> MDKYDKNVPSDYDGLFQKAADANGVSYDLLRKVAWTESRFVPTAKSKTGPLGMMQFTKATAKALGLRVTDGPDDDRLNPELAINAAAKQLAGLVGKFDGDELKAALAYNQGEGRLGNPQLEAYSKGDFASISEEGRNYMRNLLDVAKSPMAGQLETFGGITPKGKGIPAEVGLAGIGHKQKVTQELPESTSFDVKGIEQEATAKPFAKDFWETHGETLDEYNSRSTFFGFKNAAEAELSNSVAGMAFRAGRLDNGFDVFKDTITPTRWNSHIWTPEELEKIRTEVKNPAYINVVTGGSPENLDDLIKLANENFENDSRAAEAGLGAKLSAGIIGAGVDPLSYVPMVGVTGKGFKLINKALVVGAESAALNVASEGLRTSVAGGDADYAGAALGGFVFGAGMSAISDAVAAGLKRSKPEAEFDNEFIGPMMRLEARETARNANSADLSRMNTENMKFEGEHNGVPYEDLPTERGAVVLHDGSVLSASNPINPKTLKEFSEVDPEKAARGIKLAGFTEIGLKTLGSDDADIRRVAIDLVRSPTGMQSGASGKFGATASDIHERLHGTDQRTYNDLYKAMSDAMKDPEFSTGGAKMSREETRYTIYRRAALAIERPELQKALTPSERIVMDIIKRHFDTKRELMENPAIFGNTKAVSIFPESRHKGTYVPHVYDRHAKALMIQRYGAEGLQEGIARSWMNSYVSRPEVKARVDEMLKELHGVKEVTPEMVEKYAMDKAYGISHSDQFTNSSIIEENIEGLVGIENNSFLEARNLFDSDLSITMPDGQQFSVNDLRDFDMFRIMPAYDRRVNGDIAIMGSTGKTTKELKDEILALKAKAEGDGKKTGEVHALMDTVKILTGRARRNQDTVWETSLRAINDLGFFAKNAYMGAQNITEIAGMIVTGNVRALGHGIPILRDTLYKSKPVSAKELKELHASLFGKEVDQLIRPKRADIVQRLREATDTGPAVANIVGTLKYSTQELAARSPWTKLLNGTTNYLLDAARQGMLGDVISATLTGKTTRWEKEGFLRGASVTPEQMAGIKSLIKEHMVRGEDGKFTVKDKQAFSMDPRAMDLWRLADKVADEAMLRPHKVSLQDSHAFGALGKMVMQFKSFTIKSLNSKFLRTFYDGYKNNRAIDAALSIITSMGLAGGFYAMAAHVKAYALPKEKRKEYLERALDPTMIAHAALSRSSQLGAPLAMVDLVGGVLGFESSKMARSTILPKDTVKERDPNKPYTSREVMG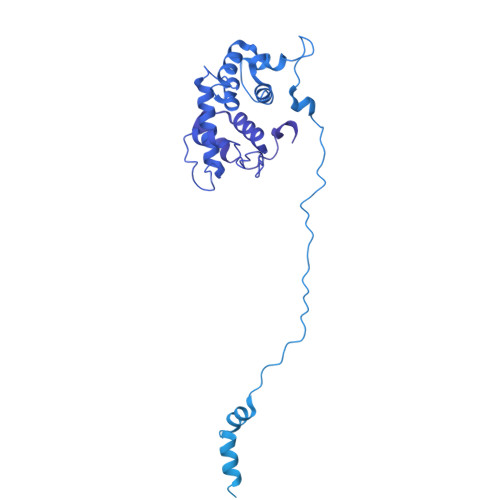AMGSNLLEQMPSAGFVANVGATLMNAAGVVNSPNKATEQDFMTGLMNSTKELVPNDPLTQQLVLKIYEANGVNLRERRK> GHMEAEVDKL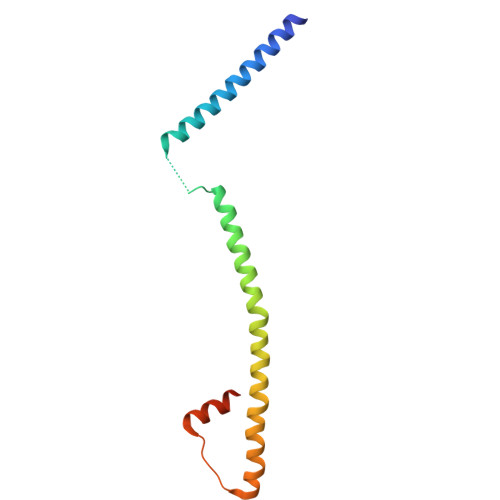ELMFQKAESDLDYIQYRLEYEIKTNHPDSASEKNPVTLLKELSVIKSRYQTLYARFKPVAVEQKESKSRICATVKKTMNMIQKLQKQTDLELSPLTKEEKTAAEQFKFHMPDL>[2x]GSGFQIPATITERYKVGRTIGDGNFAVVKECVERSTAREYALKIIKKSKCRGKEHMIQNEVSILRRVKHPNIVLLIEEMDVPTELYLVMELVKGGDLFDAITSTNKYTERDASGM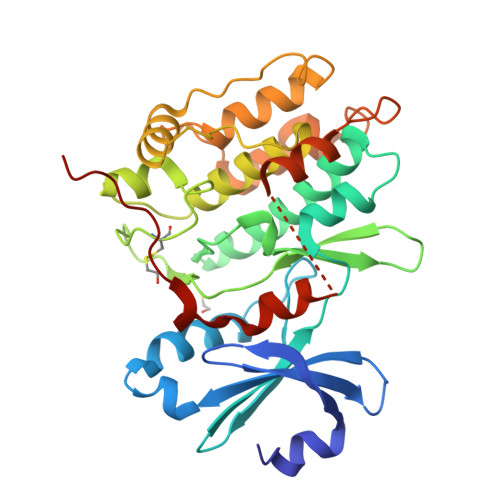LYNLASAIKYLHSLNIVHRDIKPENLLVYEHQDGSKSLKLGDFGLATIVDGPLYTVCGTPTYVAPEIIAETGYGLKVDIWAAGVITYILLCGFPPFRGSGDDQEVLFDQILMGQVDFPSPYWDNVSDSAKELITMMLLVDVDQRFSAVQVLEHPWVNDDGLPENEHQLSVAGKIKKHFNTGPKLNSTAAGVSVIATTALDKERQVFRRRRNQD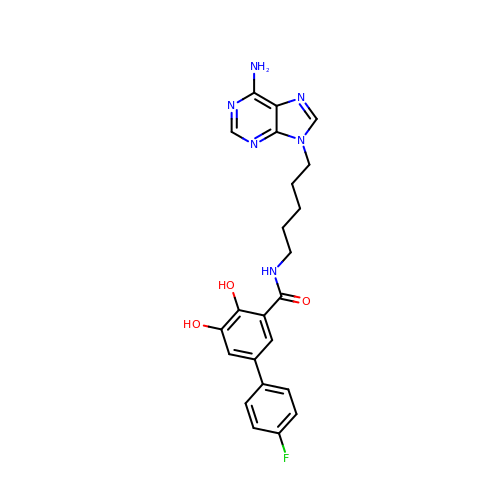N-[5-(6-aminopurin-9-yl)pentyl]-5-(4-fluorophenyl)-2,3-dihydroxybenzamide | C23 H23 F N6 O3 | CEYCKYPNLWYIGO-UHFFFAOYSA-N>[3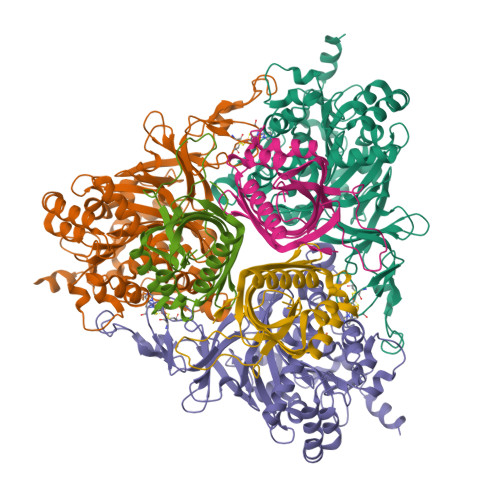x]MSSDATLVDTVNASQSRQVFWDEDVYALEIERIFSRAWLMLGHESLVPKPGDFITTYMAEDKVILSHQSDGTFRAFINSCSHRGNQICHADSGNAKAFVCNYHGWVFGQDGSLVDVPLESRCYHNSLDKQKLAAKSVRVETYKGFIFGCHDPEAPSLEDYLGEFRYYLDTIWEGAGGGMELLGPPMKSLLQCNWKVPAENFIGDGYHVGWTHAAALSQIGGELAGLAGNRADIPFDDLGLQFTTRHGHGFGVIDNAAAGLHIKREGWTKFLEDTRGEVRRKFGPERERLYLGHWNCSIFPNCSFLYGTNTFKIWHPRGPHEIEVWTYTIVPRDADPATKSMIQREAIRTFGTAGTLESDDGENMSSATYINRGVITRNGRMNSTMGVGYEGPHPVYPGIVGISFIGETSYRGFYRFWKEMIDAPDWASVKANDDTWDSVFPNRNFWNEKLNAAE;>[3x]MSSEQIPVTPDVHYDIEAHYRAEVRMFQTGQYREWLQGMVAEDIHYWMPIYEQRLTRDRRPDPTPDDAAIYNDDFGELKQRVERLYSGQVWMEDPPSKIRYFVSNVEAFEAGNGELDVLSNILVYRNRRQTEVTVHTLGREDKLRRDGNGFKVFRRKLILDARVTQDKNLYFFC>ADTIVAVELDTYPNTDIGDPSYPHIGIDIKSVRSKKTAKWNMQNGKVGTAHIIYNSVDKRLSAVVSYPNAD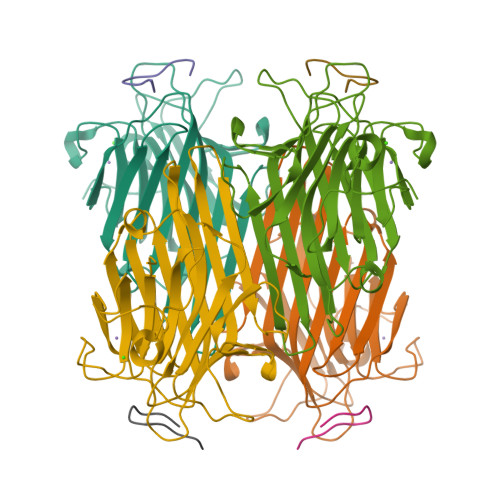SATVSYDVDLDNVLPEWVRVGLSASTGLYKETNTILSWSFTSKLKSNSTHETNALHFMFNQFSKDQKDLILQGDATTGTDGNLELTRVSSNGSPQGSSVGRALFYAPVHIWESSAVVASFEATFTFLIKSPDSHPADGIAFFISNIDSSIPSGSTGRLLGLFPDAN[4x];>MYWYPYASGS[4x]>[5x]MGNDISLIALLAFSTLLPFIIASGTCFVKFSIVFVMVRNALGLQQIPSNMTLNGVALLLSMFVMWPIMHDAYVYFEDEDVTFNDISSLSKHVDEGLDGYRDYLIKYSDRELVQFFENAQLKRQYGE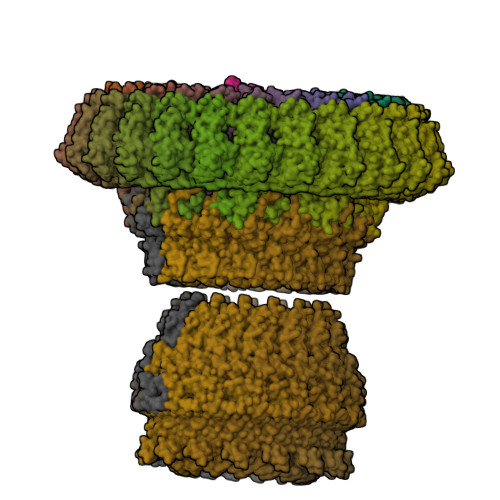ETETVKRDKDEIEKPSIFALLPAYALSEIKSAFKIGFYLYLPFVVVDLVVSSVLLALGMMMMSPVTISTPIKLVLFVALDGWTLLSKGLILQYMDIAT;> MFYALYFEIHHLVASAALGFARVAPIFFFLPFLNSGVLSGAPRNAIIILVALGVWPHALNEAPPFLSVAMIPLVLQEAAVGVMLGCLLSWPFWVMHALGCIIDNQRGATLSSSIDPANGIDTSEMANFLNMFAAVVYLQNGGLVTMVDVLNKSYQLCDPMNECTPSLPPLLTFINQVAQNALVLASPVVLVLLLSEVFLGLLSRFAPQMNAFAISLTVKSGIAVLIMLLYFSPVLPDNVLRLSFQATGLSSWFYERGATHVLE;>[4x]MDDLVFAGNKALYLVLILSGWPTIVATIIGLLVGLFQTVTQLQEQTLPFGIKLLGVCLCLFLLSGWYGEVLLSYGRQVIFLALAKG;>MKTHILLARVLACAALVLVTPGYSSEKIPVTGSGFVAKDDSLRTFFDAMALQLKEPVIVSKMAARKKITGNFEFHDPNALLEKLSLQLGLIWYFDGQAIYIYDASEMRNAVVSLRNVSLNEFNNFLKRSGLYNKNYPLRGDNRKGTFYVSGPPVYVDMVVNAATMMDKQNDGIELGRQKIGVMRLNNTFVGDRTYNLRDQKMVIPGIATAIERLLQGEEQPLGNIVSSEPPAMPAFSANGEKGKAANYAGGMSLQEALKQNAAAGNIKIVAYPDTNSLLVKGTAEQVHFIEMLVKALDVAKRHVELSLWIVDLNKSDLERLGTSWSGSITIGDKLGVSLNQSSISTLDGSRFIAAVNALEEKKQATVVSRPVLLTQENVPAIFDNNRTFYTKLIGERNVALEHVTYGTMIRVLPRFSADGQIEMSLDIEDGNDKTPQSDTTTSVDALPEVGRTLISTIARVPHGKSLLVGGYTRDANTDTVQSIPFLGKLPLIGSLFRYSSKNKSNVVRVFMIEPKEIVDPLTPDASESVNNILKQSGAWSGDDKLQKWVRVYLDRGQEAIK[16x];>[24x]MIRRYLYTFLLVMTLAGCKDKDLLKGLDQEQANEVIAVLQMHNIEANKIDSGKLGYSITVAEPDFTAAVYWIKTYQLPPRPRVEIAQMFPADSLVSSPRAEKARLYSAIEQRLEQSLQTMEGVLSARVHISYDIDAGENGRPPKPVHLSALAVYERGSPLAHQISDIKRFLKNSFADVDYDNISVVLSERSDAQLQAPGTPVKRNSFATSWIVLIILLSVMSAGFGVWYYKNHYARNKKGITADDKAKSSNE;>METSKEKTITSPGPYIVRLLNSSLNGCEFPLLTGRTLFVVGQSDALTASGQLPDIPADSFFIPLDHGGVNFEIQVDTDATEIILHELKEGNSESRSVQLNTPIQVGELLILIRPESEPWVPEQPEKLETSAKKNEPRFKNGIVAALAGFFILGIGTVGTLWILNSPQRQAAELDSLLGQEKERFQVLPGRDKMLYVAAQNERDTLWARQVLARGDYDKNARVINENEENKRISIWLDTYYPQLAYYRIHFDEPRKPVFWLSRQRNTMSKKELEVLSQKLRALMPYADSVNITLMDDVTAAGQAEAGLKQQALPYSRRNHKGGVTFVIQGALDDVEILRARQFVDSYYRTWGGRYVQFAIELKDDWLKGRSFQYGAEGYIKMSPGHWYFPSPL[24x]> GSPLPWCPHLVAVCPIPAAGLDVTQPCGDCGTIQEN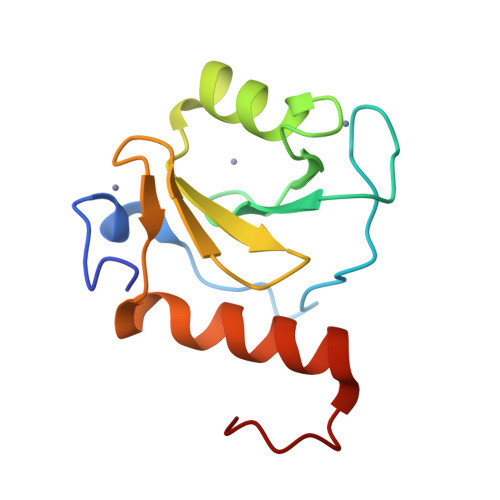WVCLSCYQVYCGRYINGHMLQHHGNSGHPLVLSYIDLSAWCYYCQAYVHHQALLDVKNIAHQNKFGEDMPHPH> GAMGSTDYNPNYCFAGKTSSISDLKEVPRKNITLIRGLGHGAFGEVYEGQVSGMPNDPSPLQVAVKTLPEVCSEQDELDFLMEALIISKFNHQNIVRCIGVSLQSLPRFILLELMAGGDLKSFLRETRPRPSQPSSLAMLDLLHVARDIACGCQYLEENHFIHRDIAARNCLLTCPGPGRVAKIGDFGMARDIYRASYYRKGGCAMLPVKWMPPEAFMEGIFTSKTDTWSFGVLLWEIFSLGYMPYPSKSNQEVLEFVTSGGRMDPPKNCPGPVYRIMTQCWQH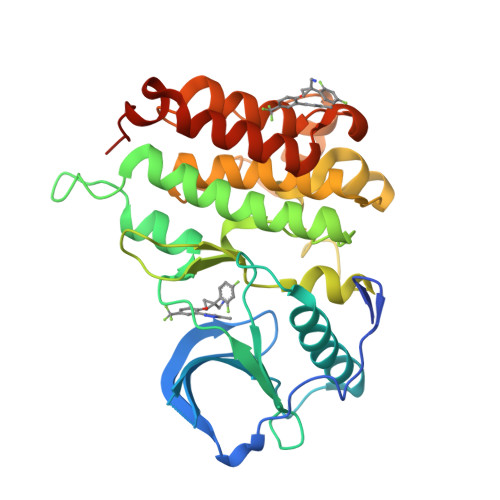QPEDRPNFAIILERIEYCTQDPDVINTALPIEYGPLVE>[5x]SMAMFYAHALGGYDENLHAFPGISSTVAND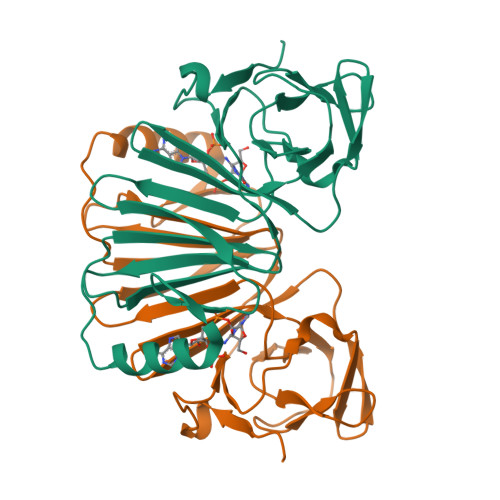VRKYSVVSVYNNKYDIVKDKYMWCYSQVNKRYIGALLPMFECNEYLQIGDPIHDQEGNQISIITYRHKNYYALSGIGYESLDLCLEGVGIHHHVLETGNAVYGKVQHDYSTIKEKAKEMNALSPGPIIDYHVWIGDCICQVTAVDVHGKEIMRMRFKKGAVLPIPNLVKVKLGENDTENLSSTISAAPSR>[3x]MNKLAVLYAEHIATLQKRTREIIERENLDGVVFHSGQAKRQFLDDMYYPFKVNPQFKAWLPVIDNP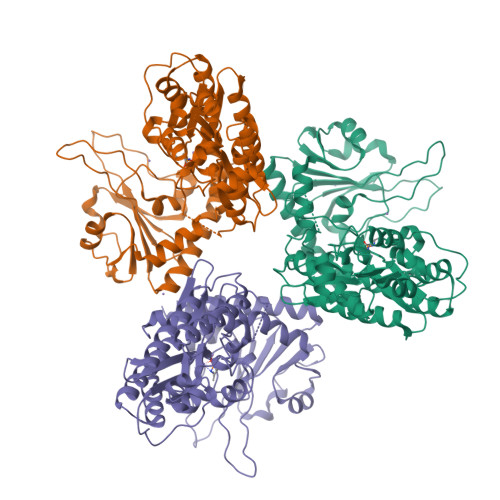HCWIVANGTDKPKLIFYRPVDFWHKVPDEPNEYWADYFDIELLVKPDQVEKLLPYDKARFAYIGEYLEVAQALGFELMNPEPVMNFYHYHRAYKTQYELACMREANKIAVQGHKAARDAFFQGKSEFEIQQAYLLATQHSENDNPYGNIVALNENCAILHYTHFDRVAPATHRSFLIDAGANFNGYAADITRTYDFTGEGEFAELVATMKQHQIALMNQLAPGKLYGELHLDCHQRVAQTLSDFNIVDLSADEIVAKGITSTFFPHGLGHHIGLQVHDVGGFMADEQGAHQEPPEGHPFLRCTRKIEANQVFTIEPGLYFIDSLLGDLAATDNNQHINWDKVAELKPFGGIRIEDNIIVHEDSLENMTRELRLRLTTHSLRGLSAPQFSINDPAVMSEYSYPSEPLSYEEEIKKSTFIVHVRTRRILVRRRTLSPILIAVTPMPAITAGLM> FSCNVDGGSSIGAGTTSVYVNLDPV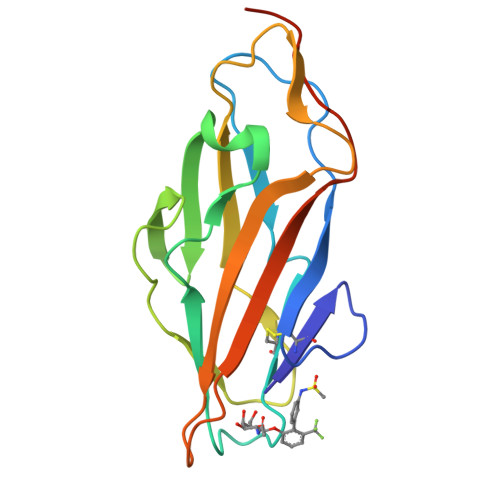IQPGQNLVVDLSQHISCWNDYGGWYDTDHINLVQGSAFAGSLQSYKGSLYWNNVTYPFPLTTNTNVLDIGDKTPMPLPLKLYITPVGAAGGVVIKAGEVIARIHMYKIATLGSGNPRNFTWNIISNNSVVMPTGGHHHHHH>MRTLITGASGQLGIELSRLLSERHEVIKVYNSSEIQGGYKLDLTDFPRLEDFIIKKRPDVIINAAAMTDVDKCEIEKEKAYKINAEAVRHIVRAGKVIDSYIVHISTDYVFDGEKGNYKEEDIPNPINYYGLSKLLGETFALQDDSLIIRTSGI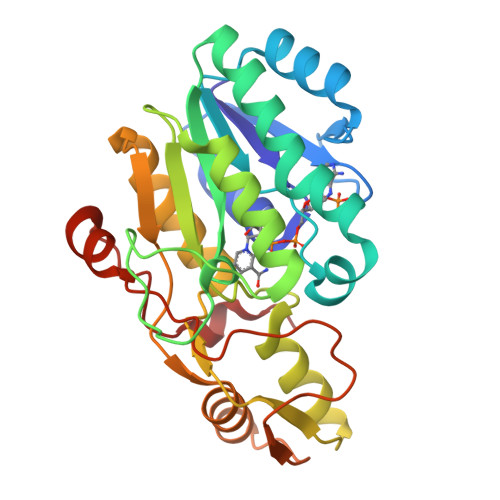FRNKGFPIYVYKTLKEGKTVFAFKGYYSPISARKLASAILELLELRKTGIIHVAGERISRFELALKIKEKFNLPGEVKEVDEVRGWIAKRPYDSSLDSSRARKILSTDFYTLDLDGMVV[2x]> TGYLTIGGQRYQAEINDLENLGEMGSG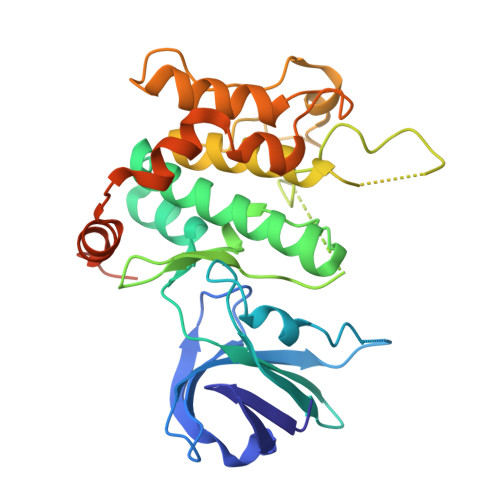TCGQVWKMRFRKTGHVIAVKQMRRSGNKEENKRILMDLDVVLKSHDCPYIVQCFGTFITNTDVFIAMELMGTCAEKLKKRMQGPIPERILGKMTVAIVKALYYLKEKHGVIHRDVKPSNILLDERGQIKLSDFGISGRLVDSKAKTRSAGCAAYMAPERIDPPDPTKPDYDIRADVWSLGISLVELATGQFPYKNCKTDFEVLTKVLQEEPPLLPGHMGFSGDFQSFVKDCLTKDHRKRPKYNKLLEHSFIKRYETLEVDVASWFKDVMAKTESPRTSGVLSQPHLPFFRHHHHHH> AATGSVTTNPTSNDEEYITQVTVGDDTLGLDFDTGSADLWVFSSQTPSSERSGHDYYTPGSSAQKIDGATWSISYGDGSSASGDVYKDKVTVGGVSYDSQAVESAEKVSSEFTQDTANDGLLGLAFSSINTVQPTPQKTFFDNVKSSLSEPIFAVALKHNAPGVYDFGYTDSSKYTGSITYTDVDNSQGFWGFTADGYSIGSDSSSDSITGIADTGTTLLLLDDSIVDAYYEQVNGASYDSSQGGYVFPSSASLPDFSVTIGDYTATVPGEYISFADVGNGQTFGGIQSNS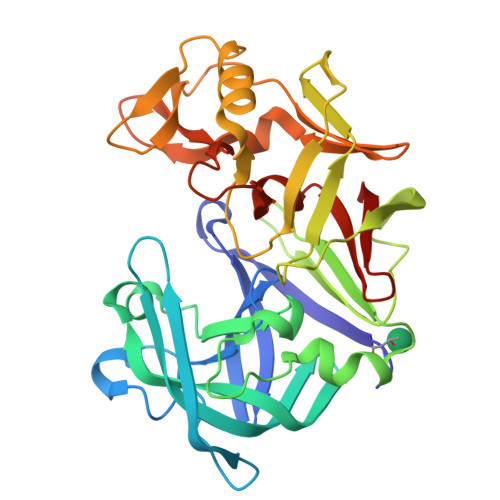GIGFSIFGDVFLKSQYVVFDASGPRLGFAAQA> MIRYLRGLVLKKEAGGFVLLAGGVGFFLQAPTPFLQALEEGKEVGVHTHLLLKEEGLSLYGFPDEENLALFELLLSVSGVGPKVALALLSALPPRLLARALLEGDARLLTSASGVGRRLAERIALEL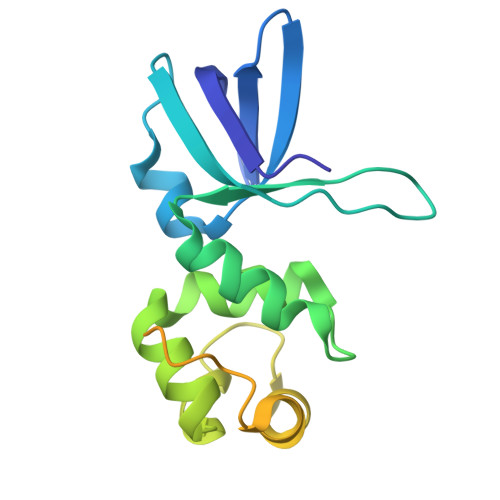KGKVPPHLLAGEKVESEAAEEAVMALAALGFKEAQARAVVLDLLAQNPKARAQDLIKEALKRLR4-[6-[bis(fluoranyl)-phenyl-methyl]-2,4-bis(oxidanylidene)-1~{H}-pyrimidin-3-yl]-5-fluoranyl-2-(2-methylphenoxy)benzenecarbonitrile 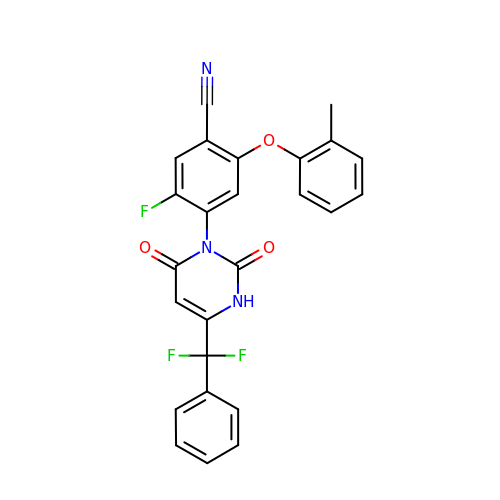| C25 H16 F3 N3 O3 | NQBGDOBAZUTXGR-UHFFFAOYSA-N>[2x]FEFPEELKTKLQEHINYFPKKRQAILLCLHEIQNYYGYIPPESLKPLADMLELPLNHVEGVVAFYDMFDREDKAKYRIRVCVSIVCHLMGTNKLLKALENILGIKPGEVTPDGKFKIVPVQCLGACSEAPVFMVNDDEYKFESEVQLNEILSRYT;>RSYPAIPRIYAETTLNMLLKRAKKPRVHSIDEYLKDGGYQALEKALNMSPEEIIDWVDKSTLRGRGGAGFPTGKKWKFAVQNPGPRYFICNADESEPGTFKDRIIIERDPHLLIEGIIISSYAIGANEAYIYIRGEYPAGYYILRDAIEEAKKKGFLGKNILGSGFDLEIYVARGAGAYICGEETALIESLEGKRGHPRLKPPYPVQKGLWGKPTVVNNVETIANVPFIISMGWEEYRYIGPSDYAGPKLFPVSGKVKKPGVYELPMNTTLREVIFKYAGGTLGNKKVKAVFSGALDCFSSEELDIPMDYSPLGFGGTGTVIVLTEEDDIVEAALKIAEFYEHETCGQCTPCRVGCYEQANLLEKIYKGEATEQDWEGFDFVNRNIQPTSICGLGAVAGRLIRQTLEKFPEEWEKYRK[2x]

Complex I couples the transfer of two electrons from NADH to ubiquinone (Q) with the translocation of four protons across the membrane. The L-shaped complex is structured into a peripheral arm that protrudes into the aqueous milieu and catalyzes electron transfer with one FMN and 8–10 iron–sulfur ([Fe–S]) clusters, and a membrane arm embedded in the lipid bilayer that mediates proton translocation. We have determined structures of the electron-input module of complex I from the hyperthermophilic bacterium Aquifex aeolicus, encompassing subunits NuoE and NuoF that contain the FMN cofactor, the [4Fe–4S] cluster N3, and the [2Fe–2S] cluster N1a, respectively, both in the air-oxidized and dithionite-reduced states at resolutions up to 1.8 Å. Here, we show that the redox state of N1a regulates NADH oxidation in complex I by inducing a conformational change close to the NADH-binding site.

To determine the mode of nucleotide binding, crystals of NuoEF were soaked with NAD+, with NADH and with NADH plus dithionite, leading to refined models at 2.0, 1.8, and 1.9 Å resolution, respectively. The structures of NADH and NADH plus dithionite-reduced NuoEF were virtually identical. Noteworthy, in the NAD+-bound state, the peptide bond between E95F and S96F faces the FMN as in the oxidized protein without nucleotide, while in the NADH-bound state, the peptide bond is pointing toward the loop coordinating N1a as it is in the structure of the reduced protein without nucleotide. Besides the atoms of ADP-ribose, all atoms of the nicotinamide ring were also clearly resolved in the structures containing NADH, while in most cases only N1 and C4 of the nicotinamide moiety are unambiguously detectable in the structures containing NAD+, indicating a dangling of the oxidized nicotinamide moiety along this molecule axis in the binding pocket. Remarkably, the reduced nicotinamide group penetrates significantly deeper into the binding pocket than its oxidized form placing it in an optimal position for hydride transfer. The amide carbon atom protrudes 1.65 Å deeper into the binding pocket changing its distance to the Cα carbon atom of Glu95F from 5.37 Å to 4.03 Å. The two positions of the nicotinamide in the binding pocket are here called tight (NADH in reduced NuoEF) and loose (NAD+ in oxidized NuoEF). Water molecules that are here resolved for the first time play an important role in substrate binding by forming hydrogen bonds between NADH and NuoF. For example, the nicotinamide N7 is bridged by a water molecule with the side chains of E95F and D103F. In NuoEF, the carbonyl group faces cluster N1a in the reduced state enabling binding of the nicotinamide in the tight position.> DYKDDDDKVPHDGNERSHRIARLAAVVSGIAGLL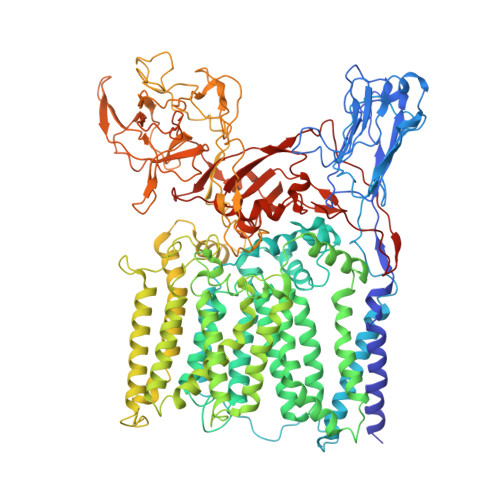LCGIVPLLPVNQTTATIFWPQGSTADGNITQITAPLVSGAPRALDISIPCSAIATLPANGGLVLSTLPAGGVDTGKAGLFVRANQDTVVVAFRDSVAAVAARSTIAAGGCSALHIWADTGGAGADFMGIPGGAGTLPPEKKPQVGGIFTDLKVGAQPGLSARVDIDTRFITTPGALKKAVMLLGVLAVLVAMVGLAALDRLSRGRTLRDWLTRYRPRVRVGFASRLADAAVIATLLLWHVIGATSSDDGYLLTVARVAPKAGYVANYYRYFGTTEAPFDWYTSVLAQLAAVSTAGVWMRLPATLAGIACWLIVSRFVLRRLGPGPGGLASNRVAVFTAGAVFLSAWLPFNNGLRPEPLIALGVLVTWVLVERSIALGRLAPAAVAIIVATLTATLAPQGLIALAPLLTGARAIAQRIRRRRATDGLLAPLAVLAAALSLITVVVFRDQTLATVAESARIKYKVGPTIAWYQDFLRYYFLTVESNVEGSMSRRFAVLVLLFCLFGVLFVLLRRGRVAGLASGPAWRLIGTTAVGLLLLTFTPTKWAVQFGAFAGLAGVLGAVTAFTFARIGLHSRRNLTLYVTALLFVLAWATSGINGWFYVGNYGVPWYDIQPVIASHPVTSMFLTLSILTGLLAAWYHFRMDYAGHTEVKDNRRNRILASTPLLVVAVIMVAGEVGSMAKAAVFRYPLYTTAKANLTALSTGLSSCAMADDVLAEPDPNAGMLQPVPGQAFGPDGPLGGISPVGFKPEGVGEDLKSDPVVSKPGLVNSDASPNKPNAAITDSAGTAGGKGPVGINGSHAALPFGLDPARTPVMGSYGENNLAATATSAWYQLPPRSPDRPLVVVSAAGAIWSYKEDGDFIYGQSLKLQWGVTGPDGRIQPLGQVFPIDIGPQPAWRNLRFPLAWAPPEADVARIVAYDPNLSPEQWFAFTPPRVPVLESLQRLIGSATPVLMDIATAANFPCQRPFSEHLGIAELPQYRILPDHKQTAASSNLWQSSSTGGPFLFTQALLRTSTIATYLRGDWYRDWGSVEQYHRLVPADQAPDAVVEEGVITVPGWGRPGPIRALP>[2x]GPLGSMTTTLANRPDGEGSVQVKLDPKVNIEEGALVIAVYGKGGIGKSTTSSNLSAAFSKLGKKVLQIGCDPKHDSTFTLTHKMVPTVIDILEEVDFHSEELRPQDFMFEGFNGVQCVESGGPPAGTGCGGYVTGQTVKLLKEHHLLEDTDVVIFDVLGDVVCGGFAAPLQHANYCLIVTANDFDSIFAMNRIVAAINAKAKNYKVRLGGVIANRSAELDQIEKFNEKTGLKTMAHFRNVDAIRRSRLKKCTIFEMDPEEEGVLEVQNEYLSLAKKMIDNVEPLEAEPLKDREIFDLLGFD;> GPLGSPEFMSGSTLLKETGPREVFCGLTSIVWLHRRMPDAFFLVVGSRTCAHLIQSAAGVMIFAEPRFGTAILEERDLAGLADAHEELDRVVKSLLKRRPEIRTLFLVGSCPSEVIKIDLSRAAERLSSQFNGQVRILNYSGSGIETTFTQGEDGALKALVPLMPSSQEEQLLLAGTLANPVEDRLKTIFNRLGIQKVESFPPRESTKLPAIGPGTKVLLAQPYLTDTARELKDRGAEILQAPFPLGVEGSQLWIEAAANAFKIKKTLVDATLEPLITRAHKALKPYVEQLSGKKLFLLPESQLEIPLARFLSNECGMKLIEVGVPYLNREMMGPELDLLPQNTRIVEGQHVEKQLDRVREHHPDLVVCGMGLANPLEAEGISTKWSIEMVFSPIHGIDQASDLAELFARPLHRQNLLNKKTLEAV;> MELTLWTYEGPPHIGAMRIATSMKGLHYVLHAPQGDTYADLLFTMIERRGSRPPVTYTTFQARDLGGDTAELVKGHIFEAVERFKPEALLVGESCTAELIQDQPGSLAKGMGLNIPIVSLELPAYSKKENWGASETFYQLIRGLLKEISEDSSNNAKQSWQEEGRRPRVNLLGPSLLGFRCRDDVLEIQKILGENGIDINVIAPLGASPSDLMRLPKADANVCLYPEIAESTCLWLERNFKTPFTKVVPIGVKATQDFLEELYELLGMEVSNSISNSDQ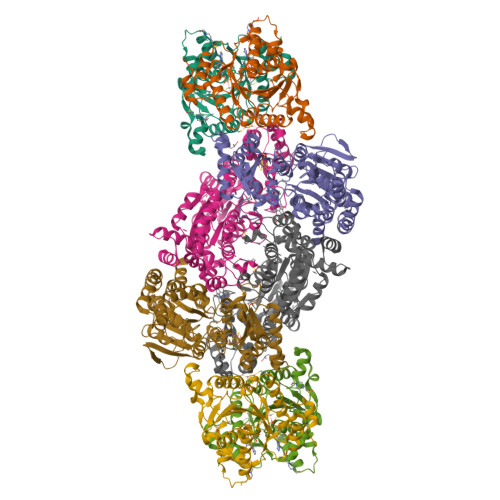SKLPWYSKSVDSNYLTGKRVFIFGDGTHVLAAARIANEELGFEVVGIGTYSREMARKVRAAATELGLEALITNDYLEVEESIKECAPELVLGTQMERHSAKRLGIPCAVISTPMHVQDVPARYSPQMGWEGANVIFDDWVHPLMMGLEEHLIGMFRHDFEFTDGHQSHLGHLGGHASETKTSSKGINQSPNNHSPAGESIHWTSEGESELAKIPFFVRGKVRRNTEKYARQAGCREIDGETLLDAKAHFGA>[2x]FLELERSSGKLEWSAILQKMASDLGFSKILFGLLPKDSQDYENAFIVGNYPAAWREHYDRAGYARVDPTVSHCT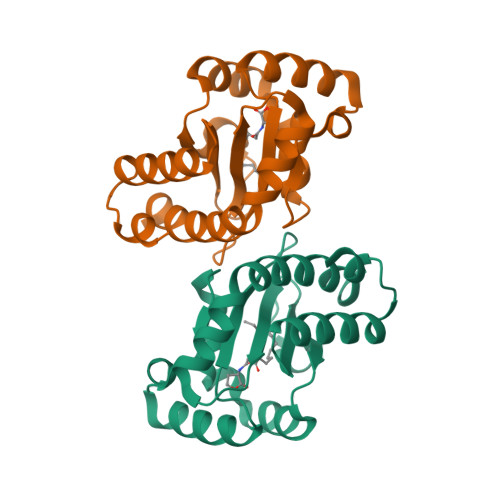QSVLPIFWEPSIYQTRKQHEFFEEASAAGLVYGLTMPLHGARGELGALSFSVEAENRAEANRFMESVLPTLWMLKDYALQSGAGLAFE> GSEGHRTLASTPALWASIPCPRSELRLDLVLPSGQSFRWREQSPAHWSGVLADQVWTLTQTEEQLHCTVYRGDKSQASRPTPDELEAVRKYFQLDVTLAQLYHHWGSVDSHFQQVAQKFQG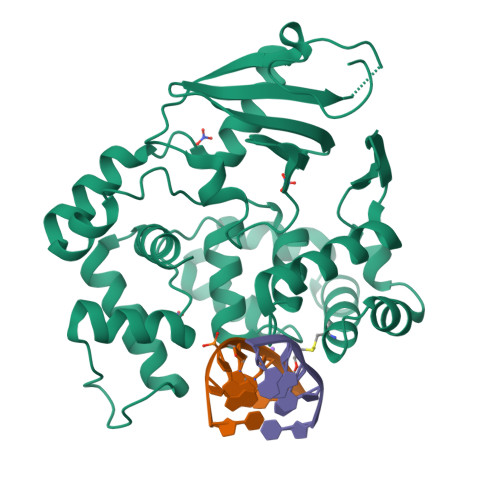VRLLRQDPIECLFSFICSSNNNIARITGMVERLCQAFGPRLIQLDDVTYHGFPSLQALAGPEVEAHLRKLGLGYRARCVSASARAILEEQGGLAWLQQLRESSYEEAHKALCILPGVGTKVADCICLMALDKPQAVPVDVHMWHIAQRDYSWHPTTSQAKGPSPQTNKELGNFFRSLWGPYAGWAQAVLFSADL> 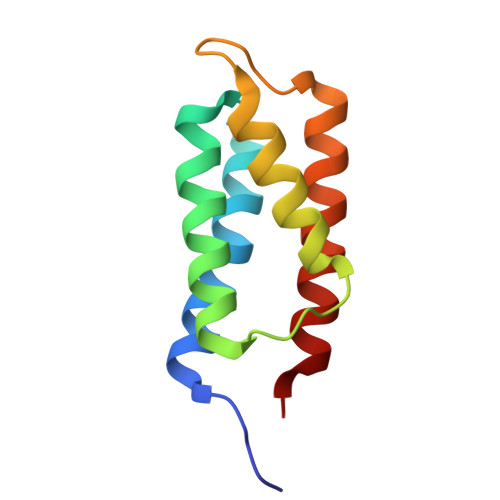HHHMFNAKYVAEATGNFITVMDALKLNYNAKDQLHPLLAELLISINRVTRDDFENRSKLIDWIVRINKLSIGDTLTETQIRELLFDLELAYKSFYALLD> MSLGAKPFGEKKFIEIKGRRMAYIDEGTGDPILFQHGNPTSSYLWRNIMPHCAGLGRLIACDLIGMGDSDKLDPSGPERYTYAEHRDYLDALWEALDLGDRVVLVVHDWGSVLGFDWARRHRERVQGIAYMEAITMPLEWADFPEQDRDLFQAFRSQAGEELVLQDNVFVEQVLPGLILRPLSEAEMAAYREPFLAAGEARRPTLSWPRQIPIAGTPADVVAIARDYAGWLSESPIPKLFINAEPGHLTTGRIRDFCRTWPNQTEITVAGAHFIQEDSPDEIGAAIAAFVRRLRPAHHH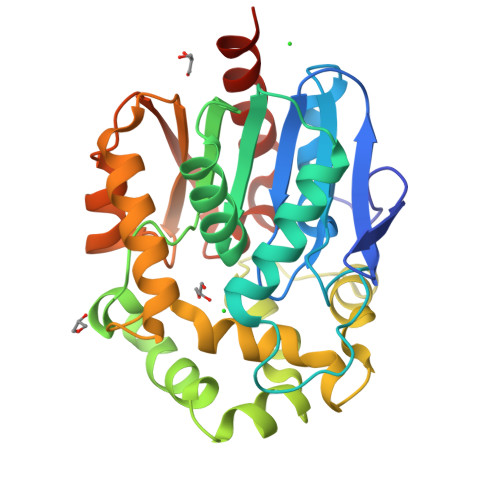HHH> EQLLPDLLISPHM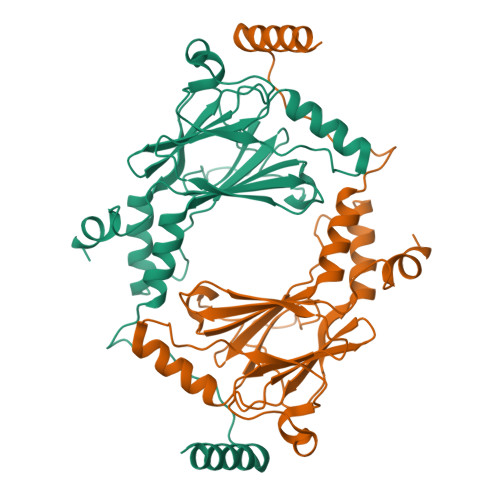LPLTDLEIKFQYRGRPPRALTISNPHGCRLFYSQLEATQEQVELFGPISLEQVRFPSPEDIPSDKQRFYTNQLLDVLDRGLILQLQGQDLYAIRLCQCKVFWSGPCASAHDSCPNPIQREVKTKLFSLEHFLNELILFQKGQTNTPPPFEIFFCFGEEWPDRKPREKKLITVQVVPVAARLLLEMFSGELSWSADDIRLQISNPDLKDRMVEQFKELHHIWQSQQRLQPVAQA>MAEFRIAQDVVARENDRRASALKEDYEALGANLARRGVDIEAVTAKVEKFFVAVPSWGVGTGGTRFARFPGTGEPRGIFDKLDDCAVIQQLTRATPNVSLHIPWDKADPKELKARGDALGLGFDAMNSNTFSDAPGQAHSYKYGSLSHTNAATRAQAVEHNLECIEIGKAIGSKALTVWIGDGSNFPGQSNFTRAFERYLSAMAEIYKGLPDDWKLFSEHKMYEPAFYSTVVQDWGTNYLIAQTLGPKAQCLVDLGHHAPNTNIEMIVARLIQFGKLGGFHFNDS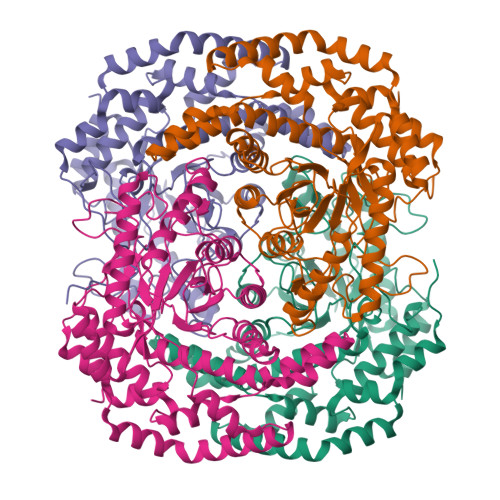KYGDDDLDAGAIEPYRLFLVFNELVDAEARGVKGFHPAHMIDQLHNVTDPIESLINSANEIRRAYAQALLVDRAALSGYQEDNDALMATETLKRAYRTDVEPILAEARRRTGGAVDPVATYRASGYRARVAAERPASVAGGGGIIGSHHHHHH[4x]>GHHHHHHELANNTTGFTRIIKAAGYSWKGLRAAWINEAAFRQEGVAVLLAVVIACWLDVDACTRVLLISSVMLVMIVELLNSAIEA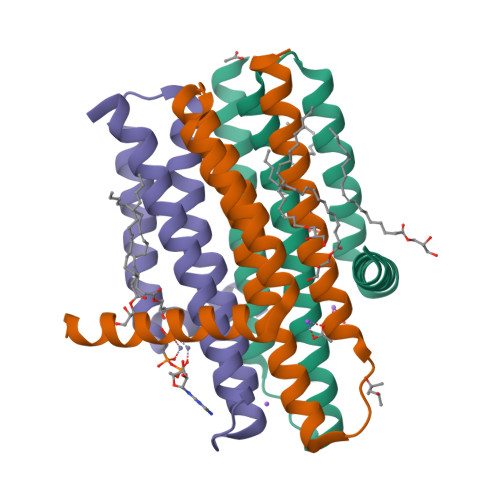VVDRIGSEYHELSGRAKDLGSAAVLIAIIDAVITWCILLWSHFG[3x]>[2x]MRYRKGARDTAFLVLYRWDLRGENPGELFKEVVEEKNIKNKDAYEYAKKLVDTAVR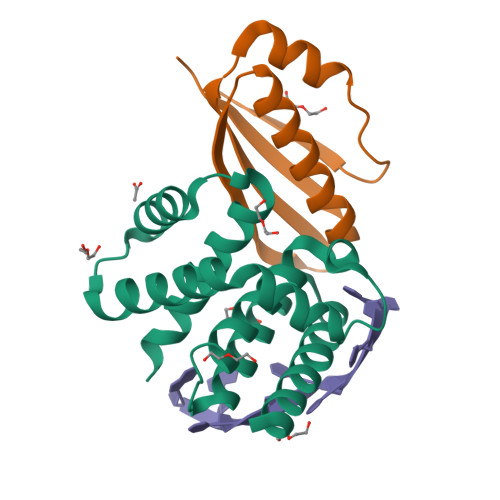HIEEIDSIIEKHLKGWSIDRLGYVERNALRLGVAELIFLKSKEPGRVFIDIVDLVKKYADEKAGKFVNGVLSAIYKAYITSSKEEKPSLKSE;>MEQEKIRIKLRAYDHRLLDQSVKQIIETVKRTGGVVKGPIPLPTRKSEFSRILDIIRFTPQTIEALMEISLPAGVDVEVKMRG[2x]>[2x]VPRGSHMKIAVMTDSTSYLSQDLIDKYNIQIAPLSVTFDDGKNFTESNEIAIEEFYNKMASSQTIPTTSQPAIGEWITKYEMLRDQGYTDIIVICLSSGISGSYQSSYQAGEMVEGVNVHAFDSKLAAMIEGCYVLRAIEMVEEGYEPQQIID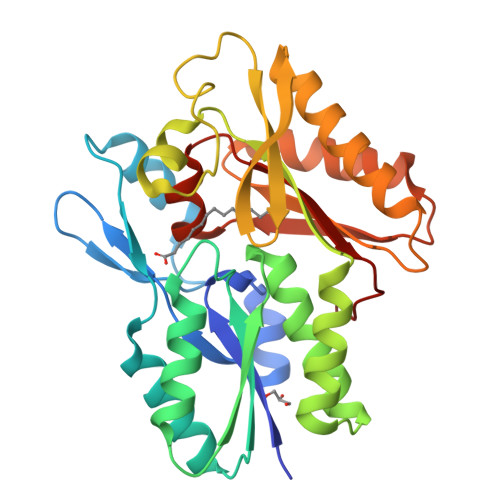DLTNMREHTGAYLIVDDLKNLQKSGRITGAQAWVGTLLKMKPVLKFEDGKIIPEEKVRTKKRAIQTLEKKVLDIVKDFEEVTLFVINGDHFEDGQALYKKLQDDCPSAYQVAYSEFGPVVAAHLGSGGLGLGYVGRKIRLT> MNDSNSLLITRLAAQILSRNMQTVDVIVDDKTLSLEEKIDTLTSMVLAVNSPPQSPPRVTSSDLAASIIKNNSKMVGNDFEMRYNVLRMAVVFVKHYPKYYNETTAGLVAEIESNLLQYQNYVNQGNYQNIEGYDSLLNKAEECYVKIDRLFKESIKKIMDDTEAFEREQEAERLRAEQTAANALLERRAQTSADDVVNRADANIPTAFSDPLPGPSAPRYMYESSESDTYMETARRTAEHYTDQDKDYNAAYTADEYNSLVKTVLLRLIEKALATLKNRLHITTIDQLKKFRDYLNSDADAGEFQIFLNQEDCVILKNLSNLASKFFNVRCVADTLEVMLEALRNNIELVQPESDAVRRIVIKMTQEIKDSSTPLYNIAMYKSDYDAIKNKNIKTLFDLYNDRLPI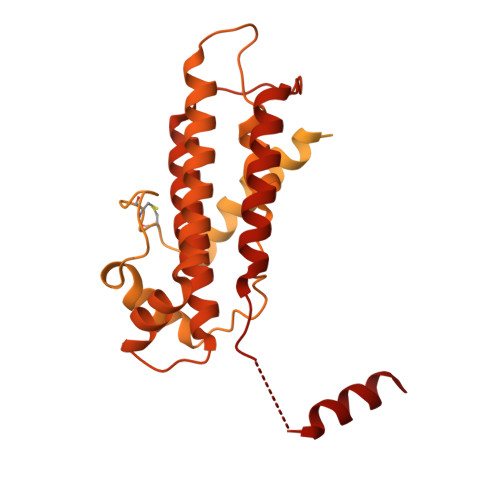NFLDTSATSPVRKTSGKRSAEDDLLPTRSSKRANRPEINVISSEDEQEDDDVEDVDYEKESKRRKLEDEDFLKLKALEFSKDIVNEKLQKIIVVTDGMKRLYEYCNCKNSLETLPSAANYGSLLKRLNLYNLDHIEMNVNFYELLFPLTLYNDNDNSDKTLSHQLVNYIFLASNYFQNCAKNFNYMRETFNVFGPFKQIDFMVMFVIKFNFLCDMRNFAKLIDELVPNKQPNMRIHSVLVMRDKIVKLAFSNLQFQTFSKKDKSRNTKHLQRLIMLMNANYNVI>HHHHHHMAKSDVKL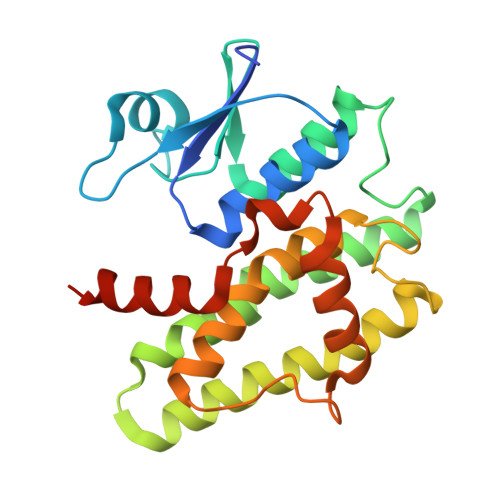LGAWPSPFVMRPRIALNIKSVEYEFLEETLGSKSQLLLESNPVHKKIPVLIHGGKPICESLVIVEYIDEVWSPGPAILPSDPYDRALARFWAAYLDEKWFPTMRNIAAAKDEEARKALIDQVGEGLVLLEDAFSKCSKGKGFFGGDQIGYLDIAFGSFLGWLRAIEKMNGVKLMDETRTPGLLKWANSFSSHPAVKDVFPETEKLVEFAKVLAKLKATPPK[4x]>MAETESIDPEKLRDQLLDAFENKQNELKSSKAYYDAERRPDAIGLAVPLDMRKYLAHVGYPRTYVDAIAERQELEGFRIPSANGEEPESGGENDPASELWDWWQANNLDIEATLGHTDALIYGTAYITISMPDPEVDFDVDPEVPLIRVEPPTALYAEVDPRTRKVLYAIRAIYGADGNEIVSATLYLPDTTMTWLRAEGEWEAPTSTPHGLEMVPVIPISNRTRLSDLYGTSEISPELRSVTDAAAQILMNMQ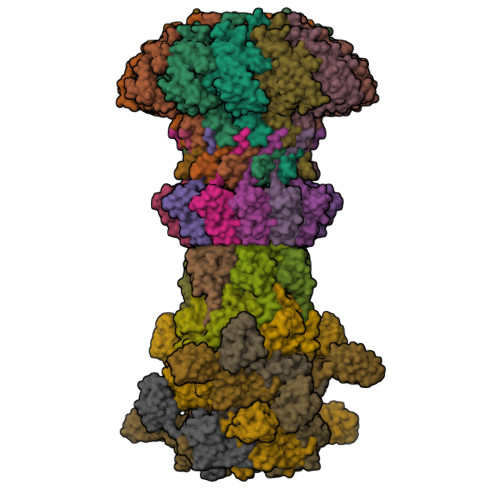GTANLMAIPQRLIFGAKPEELGINAETGQRMFDAYMARILAFEGGEGAHAEQFSAAELRNFVDALDALDRKAASYSGLPPQYLSSSSDNPASAEAIKAAESRLVKKVERKNKIFGGAWEQAMRLAYKMVKGGDIPTEYYRMETVWRDPSTPTYAAKADAAAKLFANGAGLIPRERGWVDMGYTIVEREQMRQWLEQDQKQGLGLIGSLYGASTPEGKPGEAPVGEPPAPEPDAA[12x];>[12x]MATLATHEDVTAFWARTPTAEEIVLINRRLAQAERMLLRAIPELLIKASSDPVFRAEVIDIEAEAVLRLVRNHEGYLSETDGNYTYMLQAQDPNRKLEILPEEWEVLGIVRSGLGILVPTVVLPS;>MSLLDRGGTYGSPEDGFDPVTVYPEVTRKDRLGNTLVGPSLTGIETVARFQVQGQSGTSARRAEMDDIGDMTEQVYTMRLPRSFTTELKSGSEVVWRGERWGVYGEPRRYKGSRRIAHLEYTVRRF[6x];>[6x]MAGKLPIVGEVVLPILRGHEDLSNPISTVPSLAGVHVGTWVEDIDSRTFPLITVRRVGGTRSPEHPTLFTQPVVEMTAYSAADLPTTEQMYEDALEVLYRAARLQTKTPAGYLHSVTETLGASHGPSPFDRTWRVFGLIRLGIRPPKN;>[12x]MALKDDAVLIAARGYVYTAAVGTAAPTPSQLKLIDLEHPEAWDRTGWDLVGHTSEDDLPEFGFDGGDSEVRGSWQKKKLREVETEEIADYVVINLTQFDETALELYFGPNQSATPGIFGVKSGSVVNERALLIVIVDNDVRLGFHARKASLKREDAISLATDEFGALPVRATFLDYQSYNLYEWIEEDWFNAVDAPVVYLLDLGGATGGDYTLLVGGKSTGDIAYNANASAIKTAIGAVDDGVAESAWTVTADGSDFEISGPLAVALGVDSTTGGSGVTVDVV>MSKDYMKRIQALRENYMSRRVEMDILDAYYVTQGFKATEGQPWQIQKAVAMKTVYENKPIFIQDHELLVGGVAFKPRAGILNPDSACSVIEKELDTISTRKYDPFYLSEENKKLFMEEVAPYWRGKCVLDRWNAMMPEDVRTMRDGGMLYVDKKFVRGYGENTPGWRTLLAKGITGIKKEAEEKLAALDDAHGEDVLKQIIFYKSLIISAEGIIALANRHADLAEKMAEKEADEKRRAELLKIAEVNRNVPANPPRNFYEALQSMLTYEFCIFMEQNASSYNLGRMDQYLIQYYEKDLADGTMTQDEAQELMDCFWIKISEMGLFQDGESAAFSAGYNMTVQVCAGGIDQYGNDAVNDLSYMTIQATQDTALKEPNMTVRYSISKNPDSFLRKAAECIRMGRTMPAVYHDDAGIKMLLNKGIPMSQAWDWTPCGCVETNLEGRLKSYTDIGEISMGGVVDMVMNNGRSRKTGEQISIRTGDPRDFKTFDDFMAAVKKQIDHFVHTMATMNSYLDYLSENYRPVPALSLTYPNCMAVGKDYANGGAEFNVGNGINIIGQADIINSVADIKYLVFDEKKISMDELCRALDADFEGYEHIHKMCMDAPKYGNDDPKADFCVGEIYNYLVDQIEQYDSPFGKLTAGMLPVSGNVPIGQSVGALPSGRKAWTPLADGIGATGGTDINGATALLKSISNLPHARFTQGTQMNLKIDPKLLEGERGLNSMMVLLKTQCTLDIYHTQYNVINPEILMDAQKN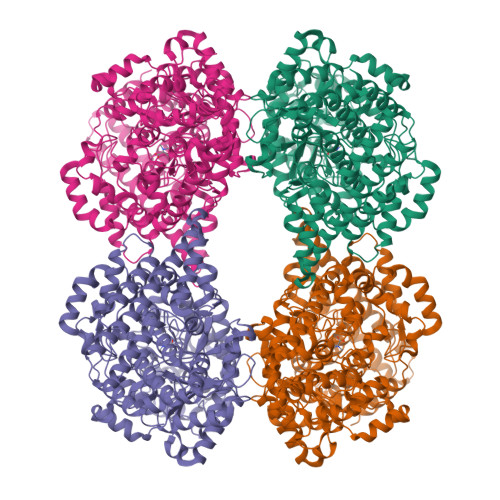PGDHKDLLVRVAGYTAFFVELGKDIQDDIIQRTEIENWG[4x]>[3x]MTPASYNLAVRRAAPAVVNVYNRGLNTNSHNQLEIR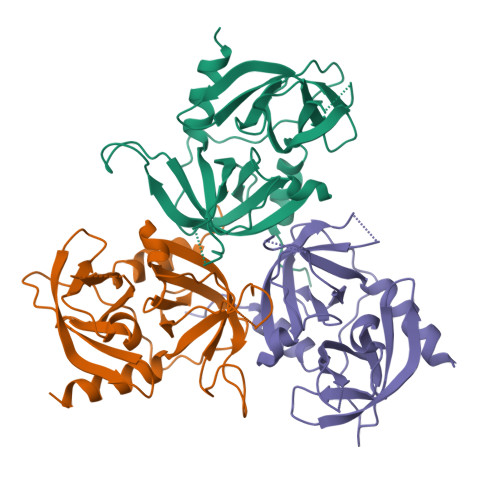TLGSGVIMDQRGYIITNKHVINDADQIIVALQDGRVFEALLVGSDSLTDLAVLKINATGGLPTIPINARRVPHIGDVVLAIGNPYNLGQTITQGIISATGRIGLNPTGRQNFLQTDASINHGNSGGALVNSLGELMGINTLSFDKSNDGETPEGIGFAIPFQLATKIMDKLIRDG>SMGWAAAREAAGRDMLAADLRCSLFASALQSYKRDSVLRPFPASYARGDCKDFEALLADASKLPNLKELLQSSGDNHKRAWDLVSWILSSKVLTIHSAGKAEFEKIQKLTGAPHTPVPAPDFLFEIEYFDPANAKFYETKGERDLIYAFHGSRLENFHSIIHNGLHCHLNKTSLFGEGTYLTSDLSLALIYSPHGHGWQHSLLGPILSCVAVCEVIDHPDVKCQTKKKDSKEIDRRRARIKHSEGGDIPPKYFVVTNNQLLRVKYLLVYSQ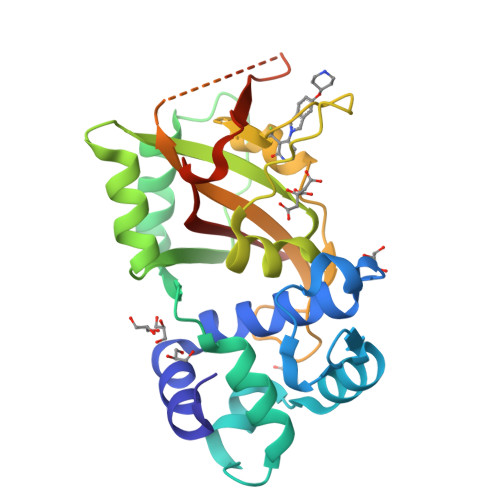KPPKRA[3x]> MVMTVRVIAPDKTVWDAPAEEVILPSTTGQLGILSNH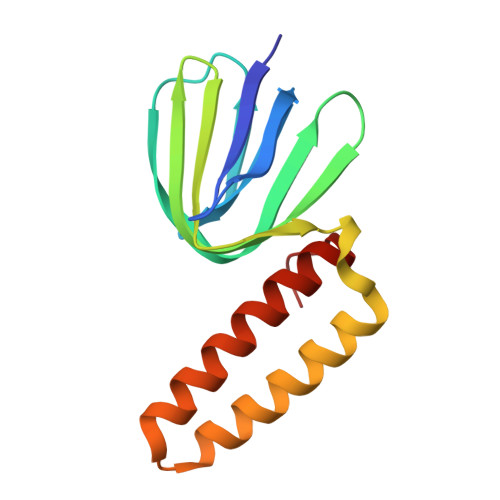APLLTALETGVMRVRQDREWVAIALMGGFAEVENNEVTILVNGAERGDTIDLEKAKAEFAAAQAALAQAEQGESKQAKIQATQAFRRARARLQAAGGVVEI>[4x]SELQTEGRTRNHGHNVCSTWGNFHYKTFDGDVFRFPGLCDYNFASDCRGSYKEFAVHLKRGPGQAEAPAGVESILLTIKDDTIYLTRHLAVLNGAVVSTPHYSPGLLIEKSDAYTKVYSRAGLTLMWNREDALMLELDTKFRNHTCGLCGDYNGLQSYSEFLSDGVLFSPLEFGNMQKINQPDVVCEDPEEEVAPASCSEHRAECERLLTAEAFADCQDLVPLEPYLRACQQDRCRCPGGDTCVCSTVAEFSRQCSHAGGRPGNWRTATLCPKTCPGNLVYLESGSPCMDTCSHLEVSSLCEEHRMDGCFCPEGTVYDDIGDSGCVPVSQCHCRLHGHLYTPGQEITNDCEQCVCNAGRWVCKDLPCPGTCALEGGSHITTFDGKTYTFHGDCYYVLAKGDHNDSYALLGELAPCGSTDKQTCLKTVVLLADKKKNVVVFKSDGSVLLNELQVNLPHVTASFSVFRPSSYHIMVSMAIGVRLQVQLAPVMQLFVTLDQASQGQVQGLCGNFNGLEGDDFKTASGLVEATGAGFANTWKAQSSCHDKLDWLDDPCSLNIESANYAEHWCSLLKKTETPFGRCHSAVDPAEYYKRCKYDTCNCQNNEDCLCAALSSYARACTAKGVMLWGWREHVCNKDVGSCPNSQVFLYNLTTCQQTCRSLSEADSHCLEGFAPVDGCGCPDHTFLDEKGRCVPLAKCSCYHRGLYLEAGDVVVRQEERCVCRDGRLHCRQIRLIGQSCTAPKIHMDCSNLTALATSKPRALSCQTLAAGYYHTECVSGCVCPDGLMDDGRGGCVVEKECPCVHNNDLYSSGAKIKVDCNTCTCKRGRWVCTQAVCHGTCSIYGSGHYITFDGKYYDFDGHCSYVAVQDYCGQNSSLGSFSIITENVPCGTTGVTCSKAIKIFMGRTELKLEDKHRVVIQRDEGHHVAYTTREVGQYLVVESSTGIIVIWDKRTTVFIKLAPSYKGTVCGLCGNFDHRSNNDFTTRDHMVVSSELDFGNSWKEAPTCPDVSTNPEPCSLNPHRRSWAEKQCSILKSSVFSICHSKVDPKPFYEACVHDSCSCDTGGDCECFCSAVASYAQECTKEGACVFWRTPDLCPIFCDYYNPPHECEWHYEPCGNRSFETCRTINGIHSNISVSYLEGCYPRCPKDRPIYEEDLKKCVTADKCGCYVEDTHYPPGASVPTEETCKSCVCTNSSQVVCRPEEGKILNQTQDGAFCYWEICGPNGTVEKHFNICSITHHHHHH

One extracellular protein family that arose through domain replication and gene duplication is the gel-forming mucins, huge glycoproteins that coat and protect the epithelia in the lungs, intestines, and other organs. A remarkable variation on the theme of mucins arose with the evolution of the complex vasculature in the vertebrate lineage. von Willebrand factor (VWF), a glycoprotein responsible for hemostasis, has a similar domain organization and is homologous to mucins in its amino- and carboxyl-terminal regions. Under acidic conditions, the amino termini of mucins and VWF form noncovalent intermolecular interactions that juxtapose VWD3 assemblies from different CTCK-linked dimers. We present residue-resolution structures of VWF and MUC2 amino-terminal segment tubules, enabling comparison between them and an analysis of the features that stabilize each one.

We subsequently discovered using dynamic light scattering (DLS) that a dimeric MUC2 amino-terminal fragment spanning the D1D2D3 region but lacking CysD1 could also self-assemble, but only at a lower pH. Remarkably, in TEM samples prepared at pH 5.4, the D1D2D3 fragment exhibited tubules that resembled the VWF tubules found in WPBs, both with diameters of ∼25 nm. The VWF and MUC2 tubules also both display twofold symmetry perpendicular to the helix axis. They differ, however, in that the VWF tubule is a one-start helix, whereas the MUC2 tubule is a two-start helix. The MUC2 tubule has a helical twist of ∼83.2° (about 4.3 subunits per turn) and an axial rise of ∼6.95 nm per subunit. The MUC2 subregion map also consisted of two adjacent beads at a nominal resolution of 3.4 Å, but one bead appeared at higher resolution than the second. The resolution difference between the beads in the MUC2 map may indicate greater flexibility between beads compared to the VWF tubule. The recombinant MUC2 D1D2D3 segment used for tubule assembly in this study was intact. Nevertheless, the MUC2 E2-TIL′ junction was also unresolved, suggesting that it is a flexible joint. In contrast, apposing MUC2 D2 domains appear only very weakly associated in the tubule (Right). Additionally, interactions are not evident in the MUC2 tubule between the bridge and D1 or D2.> MEYRMFDIGVNLTSSQFAKDRDDVVACAFDAG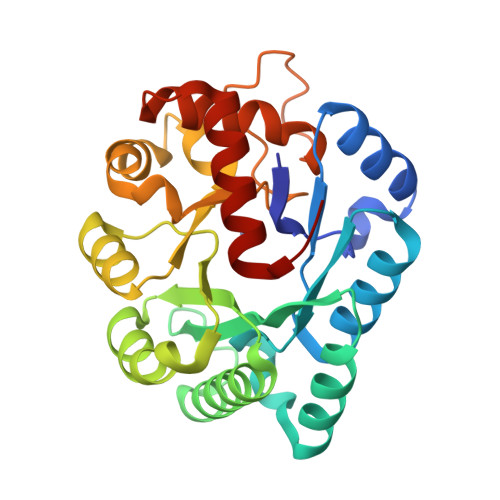VNGLLITGTNLRESQQAQKLARQYSSCWSTAGVHPHDSSQWQAATEEAIIELAAQPEVVAIGECGLDFNRNFSTPEEQERAFVAQLRIAADLNMPVFMHCRDAHERFMTLLEPWLDKLPGAVLHCFTGTREEMQACVAHGIYIGITGWVCDERRGLELRELLPLIPAEKLLIETDAPYLLPRDLTPKPSSRRNEPAHLPHILQRIAHWRGEDAAWLAATTDANVKTLFGIAF> IVGGYTCAANSIPYQVSLNSGSHFCGGSLINSQWVVSAAHCYKSRIQVRLGEHNIDVLEGNEQFINAAKIITHPNFNGNTLDNDIMLIKLSSPATLNSRVATVSLPRSCAAAGTECLISGWGNTKSSGSSYPSLLQCLKAPVLSDSSCKSSYPGQITGNMICVGFLEGGKDSCQGDSGGPVVCNGQLQGIVSWGYGCAQKNKPGVYTKVCNYVNWIQQTIAAN;> 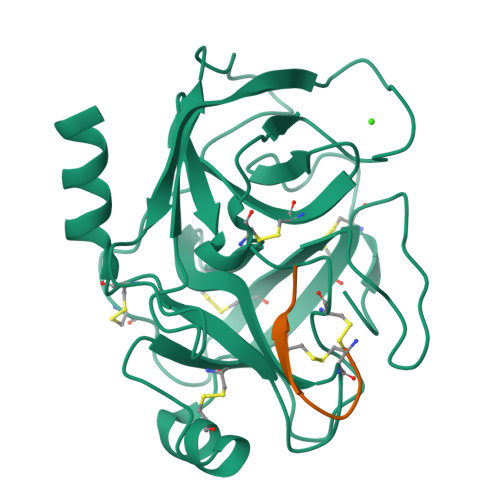CYFQNCPRGX N-(4-bromophenyl)-2-[2-(1,3-thiazol-2-yl)-1H-benzimidazol-1-yl]acetamide | C18 H13 Br N4 O S | 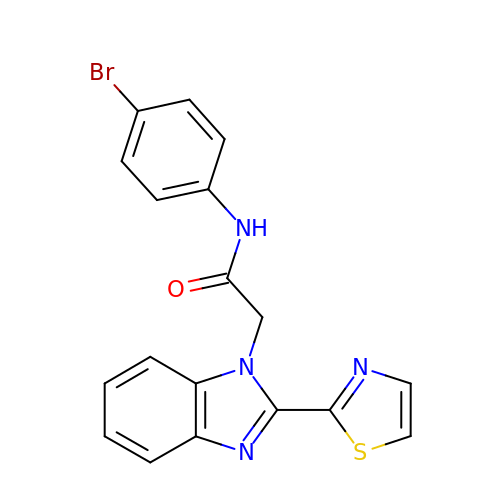GUHIASUSWSGRHY-UHFFFAOYSA-N> SNAMAKTLKDLQGWEIITTDEQGNIIDGGQKRLRRRGAKTEHYLKRSSDGIKLGRGDSVVMHNEAAGTYSVYMIQELRLNTLNNVVELWALTYLRWFEVNPLAHYRQFNPDANILNRPLNYYNKLFSETANKNELYLTAELAELQLFNFIRVANVMDGSKWEVLKGNVDPERDFTVRYICEPTGEKFVDINIEDVKAYIKKVEPREAQEYLKDLTLPSKKKEIKRGPQKKDKATQTAQISDAETRATDITDNEDGNEDESSDYESPSDIDVSEDMDSGEISADELEEEEDEEEDEDEEEKEARHTNSPRKRGRKIKLGKDDIDASVQPPPKKRGRKPKDPSKPRQMLLISSCRANNTPVIRKFTKKNVARAKKKYTPFSKRFKSIAAIPDLTSLPEFYGNSSELMASRFENKLKTTQKHQIVETIFSKVKKQLNSSYVKEEILKSANFQDYLPARENEFASIYLSAYSAIESDSATTIYVAGTPGVGKTLTVREVVKELLSSSAQREIPDFLYVEINGLKMVKPTDCYETLWNKVSGERLTWAASMESLEFYFKRVPKNKKKTIVVLLDELDAMVTKSQDIMYNFFNWTTYENAKLIVIAVANTMDLPERQLGNKITSRIGFTRIMFTGYTHEELKNIIDLRLKGLNDSFFYVDTKTGNAILIDAAGNDTTVKQTLPEDVRKVRLRMSADAIEIASRKVASVSGDARRALKVCKRAAEIAEKHYMAKHGYGYDGKTVIEDENEEQIYDDEDKDLIESNKAKDDNDDDDDNDGVQTVHITHVMKALNETLNSHVITFMTRLSFTAKLFIYALLNLMKKNGSQEQELGDIVDEIKLLIEVNGSNKFVMEIAKTLFQQGSDNISEQLRIISWDFVLNQLLDAGILFKQTMKNDRICCVKLNISVEEAKRAMNEDETLRNL;> MLNGEDFVEHNDILSSPAKSRNVTPKRVDPHGERQLRRIHSSKKNLLERISLVGNERKNTSPDPALKPKTPSKAPRKRGRPRKIQEELTDRIKKDEKDTISSKKKRKLDKDTSGNVNEESKTSNNKQVMEKTGIKEKREREKIQVATTTYEDNVTPQTDDNFVSNSPEPPEPATPSKKSLTTNHDFTSPLKQIIMNNLKEYKDSTSPGKLTLSRNFTPTPVPKNKKLYQTSETKSASSFLDTFEGYFDQRKIVRTNAKSRHTMSMAPDVTREEFSLVSNFFNENFQKRPRQKLFEIQKKMFPQYWFELTQGFSLLFYGVGSKRNFLEEFAIDYLSPKIAYSQLAYENELQQNKPVNSIPCLILNGYNPSCNYRDVFKEITDLLVPAELTRSETKYWGNHVILQIQKMIDFYKNQPLDIKLILVVHNLDGPSIRKNTFQTMLSFLSVIRQIAIVASTDHIYAPLLWDNMKAQNYNFVFHDISNFEPSTVESTFQDVMKMGKSDTSSGAEGAKYVLQSLTVNSKKMYKLLIETQMQNMGNLSANTGPKRGTQRTGVELKLFNHLCAADFIASNEIALRSMLREFIEHKMANITKNNSGMEIIWVPYTYAELEKLLKTVLNTL;> MSDLNQSKKMNVSEFADAQRSHYTVYPSLPQSNKNDKHIPFVKLLSGKESEVNVEKRWELYHQLHSHFHDQVDHIIDNIEADLKAEISDLLYSETTQKRRCFNTIFLLGSDSTTKIELKDESSRYNVLIELTPKESPNVRMMLRRSMYKLYSAADAEEHPTIKYEDINDEDGDFTEQNNDVSYDLSLVENFKRLFGKDLAMVFNFKDVDSINFNTLDNFIILLKSAFKYDHVKISLIFNINTNLSNIEKNLRQSTIRLLKRNYHKLDVSSNKGFKYGNQIFQSFLDTVDGKLNLSDRFVEFILSKMANNTNHNLQLLTKMLDYSLMSYFFQNAFSVFIDPVNVDFLNDDYLKILSRCPTFMFFVEGLIKQHAPADEILSLLTNKNRGLEEFFVEFLVRENPINGHAKFVARFLEEELNITNFNLIELYHNLLIGKLDSYLDRWSACKEYKDRLHFEPIDTIFQELFTLDNRSGLLTQSIFPSYKSNIEDNLLSWEQVLPSLDKENYDTLSGDLDKIMAPVLGQLFKLYREANMTINIYDFYIAFRETLPKEEILNFIRKDPSNTKLLELAETPDAFDKVALILFMQAIFAFENMGLIKFQSTKSYDLVEKCVWRGI;> SNAMTISEARLSPQVNLLPIKRHSNEEVEETAAILKKRTIDNEKCKDSDPGFGSLQRRLLQQLYGTLPTDEKIIFTYLQDCQQEIDRIIKQSIIQKESHSVILVGPRQSYKTYLLDYELSLLQQSYKEQFITIRLNGFIHSEQTAINGIATQLEQQLQKIHGSEEKIDDTSLETISSGSLTEVFEKILLLLDSTTKTRNEDSGEVDRESITKITVVFIFDEIDTFAGPVRQTLLYNLFDMVEHSRVPVCIFGCTTKLNILEYLEKRVKSRFSQRVIYMPQIQNLDDMVDAVRNLLTVRSEISPWVSQWNETLEKELSDPRSNLNRHIRMNFETFRSLPTLKNSIIPLVATSKNFGSLCTAIKSCSFLDIYNKNQLSNNLTGRLQSLSDLELAILISAARVALRAKDGSFNFNLAYAEYEKMIKAINSRIPTVAPTTNVGTGQSTFSIDNTIKLWLKKDVKNVWENLVQLDFFTEKSAVGLRDNATAAFYASNYQFQGTMIPFDLRSYQMQIILQELRRIIPKSNMYYSWTQL;> MNVTTPEVAFREYQTNCLASYISADPDITPSNLILQGYSGTGKTYTLKKYFNANPNLHAVWLEPVELVSWKPLLQAIARTVQYKLKTLYPNIPTTDYDPLQVEEPFLLVKTLHNIFVQYESLQEKTCLFLILDGFDSLQDLDAALFNKYIKLNELLPKDSKINIKFIYTMLETSFLQRYSTHCIPTVMFPRYNVDEVSTILVMSRCGELMEDSCLRKRIIEEQITDCTDDQFQNVAANFIHLIVQAFHSYTGNDIFALNDLIDFKWPKYVSRITKENIFEPLALYKSAIKLFLSTDDNLSENGQGESAITTNRDDLENSQTYDLSIISKYLLIASYICSYLEPRYDASIFSRKTRIIQGRAAYGRRKKKEVNPRYLQPSLFAIERLLAIFQAIFPIQGKAESGSLSALREESLMKANIEVFQNLSELHTLKLIATTMNKNIDYLSPKVRWKVNVPWEIIKEISESVHFNISDYFSDIHE;> MSMQQVQHCVAEVLRLDPQEKPDWSSGYLKKLTNATSILYNTSLNKVMLKQDEEVARCHICAYIASQKMNEKHMPDLCYYIDSIPLEPKKAKHLMNLFRQSLSNSSPMKQFAWTPSPKKNKRSPVKNGGRFTSSDPKELRNQLFGTPTKVRKSQNNDSFVIPELPPMQTNESPSITRRKLAFEEDEDEDEEEPGNDGLSLKSHSNKSITGTRNVDSDEYENHESDPTSEEEPLGVQESRSGRTKQNKAVGKPQSELKTAKALRKRGRIPNSLLVKKYCKMTTEEIIRLCNDFELPREVAYKIVDEYNINASRLVCPWQLVCGLVLNCTFIVFNERRRKDPRIDHFIVSKMCSLMLTSKVDDVIECVKLVKELIIGEKWFRDLQIRYDDFDGIRYDEIIFRKLGSMLQTTNILVTDDQYNIWKKRIEMDLALTEPL;> SNAMSAIPITPTKRIRRNLFDDAPATPPRPLKRKKLQFTDVTPESSPEKLQFGSQSIFLRTKALLQKSSELVNLNSSDGALPARTAEYEQVMNFLAKAISEHRSDSLYITGPPGTGKTAQLDMIIRQKFQSLPLSLSTPRSKDVLRHTNPNLQNLSWFELPDGRLESVAVTSINCISLGEPSSIFQKIFDSFQDLNGPTLQIKNMQHLQKFLEPYHKKTTFVVVLDEMDRLLHANTSETQSVRTILELFLLAKLPTVSFVLIGMANSLDMKDRFLSRLNLDRGLLPQTIVFQPYTAEQMYEIVIQKMSSLPTIIFQPMAIKFAAKKCAGNTGDLRKLFDVLRGSIEIYELEKRFLLSPTRGSLNSAQVPLTPTTSPVKKSYPEPQGKIGLNYIAKVFSKFVNNNSTRTRIAKLNIQQKLILCTIIQSLKLNSDATIDESFDHYIKAITKTDTLAPLQRNEFLEICTILETCGLVSIKKTKCKGKTKRFVDKIDVDLDMREFYDEMTKISILKPFLH

The coordinated action of multiple replicative helicase loading factors is needed for the licensing of replication origins prior to DNA replication. Binding of the Origin Recognition Complex (ORC) to DNA initiates the ATP-dependent recruitment of Cdc6, Cdt1 and Mcm2-7 loading, but the structural details for timely ATPase site regulation and for how loading can be impeded by inhibitory signals, such as cyclin-dependent kinase phosphorylation, are unknown. Apart from Cdt1 and Orc6 (a subunit of ORC), all loading factors belong to the superfamily of ATPases Associated with various cellular Activities (AAA+). Here, we report cryo-EM structures of ARS1-bound S. cerevisiae (Sc) ORC and of the ternary complex with Cdc6 at sub-3 Å resolutions.

In our cryo-EM structure of the ternary complex, Cdc6 is seen to complete the ORC ring as expected by binding in between Orc1 and Orc2. Surprisingly, masked classification of the Cdc6 region revealed that the ORC·Cdc6 ring adopts two distinct conformations that differ in pitch and the positioning of Cdc6. The two states arise from a rocking motion of mainly Orc1 and Cdc6, which leads to ring flattening as the complex transitions from state 1 to state 2 (referred to as ODC1 and ODC2 hereafter). Both states also differ from the ring conformation seen in a loading intermediate containing DNA, ORC, Cdc6, Cdt1, and Mcm2-7 (OCCM), indicating this change in ring conformation may be linked to the functional ORC·Cdc6 cycle during Mcm2-7 loading. One possibility is that Cdc6 binding drives ScORC into a hydrolysis-competent conformation; however, inspection of the Orc1·Orc4 ATPase site configuration in our 2.5 and 2.7 Å cryo-EM structures of ODC1 and ODC2 reveals that the active site waters remain in a non-lytic position. The Orc1-sensor 1 is also flipped away from ATP in ODC1, although it appears to move closer to ATP in ODC2. The second ATPase center in the ternary ScORC·DNA·Cdc6 complex at the interface between Orc1 and Cdc6 likewise appears to reside in a pre-hydrolysis state. Overall, the Cdc6·Orc1 sites in ODC1 and ODC2 are configured very similarly to each other and to that of Orc1 and Orc4, but the Cdc6-sensor 1 (N263), which is important for budding yeast viability and ATP hydrolysis by Cdc648,58,59, points into the active site and bonds with the γ-phosphate. A water molecule positioned for an in-line nucleophilic attack, however, is not seen. Intriguingly, Cdc6 binding to ScORC causes conformational rearrangements in the B-loop of Orc1 that help reorient the Orc1 arginine finger helix (with arginine finger R616) for completion of the Cdc6 ATPase site.In cells, GCs bind to the glucocorticoid receptor (GR), a steroid hormone nuclear receptor that regulates the expression of thousands of genes. GC binding to the GR ligand binding domain (LBD) in the cytoplasm causes it to translocate to the nucleus where its DNA binding domain (DBD) recognizes and binds to specific GR DNA binding sequences (GBSs) or inverted repeat GBSs (IR-GBSs). In fact, crystal structures of GR DBD bound to various GBSs revealed a loop region in the DBD, the lever arm between the DNA recognition helix and the dimerization loop, whose conformation is sensitive to the bound DNA’s sequence. Here, we have solved the crystal structure of the GR DBD in its DNA-free state.

The GR DBD crystallized in its free form in space group P1 with eight molecules in the asymmetric unit. The eight molecules contain four dimers that are linked by a disulfide bridge via Cys431. While this dimer appears to be advantageous for crystallization (no reducing agents were present during crystallization) it is not likely to form under physiological conditions in the intracellular reducing environment. Within each dimer, one molecule shows clear density within the C-terminal helix (H3) following the core DBD, whereas this stretch is mostly disordered in the other molecule. In the free state observed here, H3 is rotated by approximately 60 degrees so that it would lie across the minor groove of a bound DNA. However, the current structure suggests that the orientation of H3 relative to the core DBD is not fixed in the absence of DNA and adopts its active conformation only upon GR binding to a recognition sequence. The core DBD (residues 421–491) of the individual molecules within the unit cell are very similar in structure (average pairwise RMSD = 0.49 Å). The largest differences are located within the lever arm region and are similar in extent to the variations observed in GR DBD bound to different GBSs. In the free crystal structure, His453 is flipped out in all molecules. However, close inspection of electron density shows evidence for an alternative, packed conformation in four molecules. These observations suggest that the lever arm, including His453, is mobile in the free state and samples multiple conformations resembling the various structures in the presence of different DNA sequences.

>SPKLCLVCSDEASGCHYGVLTCGSCKVFFKRAVEGQHNYLCAGRNDCIIDKIRRKNCPACRYRKCLQAGMNLEARKTKKKIKGIQQATTG[8x]>LQALLPKAQSVGNSRVRFTTAEVDSAVARISQKIGVPASYYQFLIPIENFVVAGGFETTVS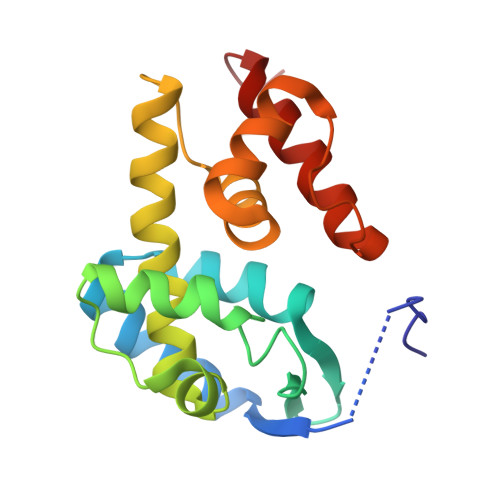GSFRGLGQFNRQTWDGLRRLGRNLPAFEEGSAQLNASLYAIGFLYLENKRAYEASFKGRVFTHEIAYLYHNQGAPAAEQYLTSGRLVYPKQSEAAVAAFAAARNQHVKESWA[2x]>[7x]MANMQGGQRLGTNQGKGQSAADKLALFLKVFGGEVLTAFARTSVTTNRHMQRQISSGKSAQFPVIGRTKAAYLQPGESLDDKRKD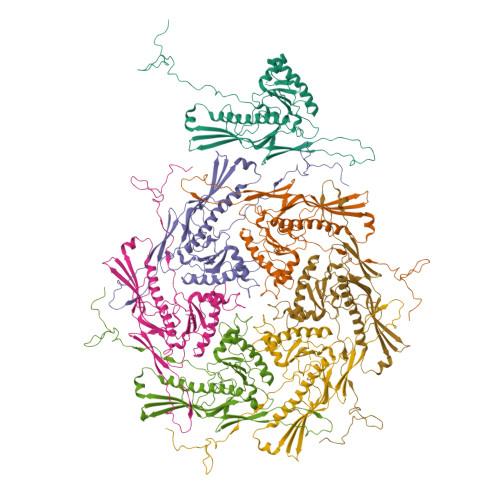IKHTEKTINIDGLLTADVLIYDIEDAMNHYDVRSEYTSQIGESLAMAADGAVLAELAGLVNLADSVNENIAGLGKPSLLEVGLKADLTDPVKLGQAVIAQLTIARAALTKNYVPANDRTFYTTPDVYSAILAALMPNAANYAALIDPERGSIRNVMGFEVVEVPHLTAGGAGDDRPDEGAEATNQKHAFPAAGGKVNKENVVGLFQHRSAVGTVKLKDLALERARRTEYQADQIVAKYAMGHGGLRPESAGALVFTAASA>MTPNWSELVAAADPALVLPSGERRAEVAVPGPLRLDALLDLGEGHAVGVVRSADAARWTVPLVRDGAGGVRRSRPGDGTAEHLVAALARRGATPDAAFVLEAFTGAAPVTGERGIIVDQTNESVIVGECAVVKWAVRLPAEGEPGSPAAQRIAALARGGFTEMPRPWGLLTLAEGAQPVLLASVVAYLPGALDGWDWAVDDVRRLARGELTMDQALLPAAQLGTLTARMHAALAARGRTPATAADVAAWGVRMREELDEAVASVPGAEGERLKAWAPRIADVYAELDALAGTPLIDVHGDFHVGQILRADGRYAVVDFDGNPVLPADQRAARQPAAL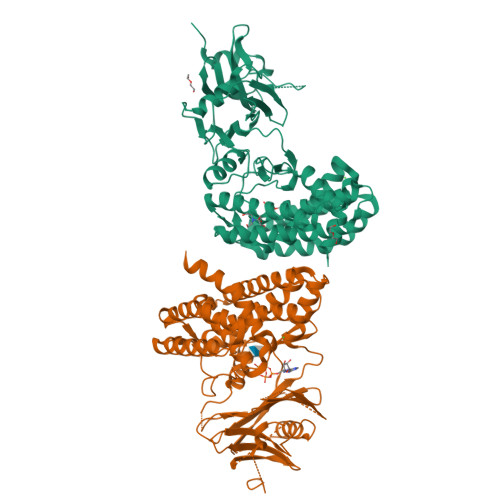DVVGMTASLDHVGRVVVFRTPDVDPAPVRAWIAAAQRSFLDAYRTTLARLDADDLFDDRLLTPLRYAQEVREYLYAVRHLPHWVYVPDLSLTDLLPERLKDKLAAALEHHHHHH[2x]> YEYVELAKASLTSAQPQHFYAVVIDATFPYKTNQERYICSLKIVDPTLYLKQQKGAGDASDYATLVLYAKRFEDLPIIHRAGD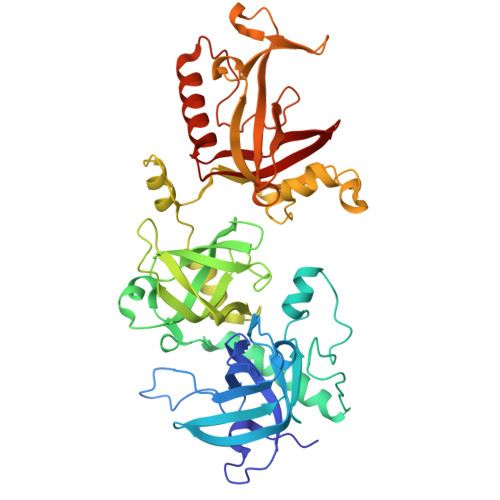IIRVHRATLRLYNGQRQFNANVFYSSSWALFSTDKRSVTQEINNQDAVSDTTPFSFSSKHATIEKNEISILQNLRKWANQYFSSYSVISSDMYTALNKAQAQKGDFDVVAKILQVHELDEYTNELKLKDASGQVFYTLSLKLKFPHVRTGEVVRIRSATYDETSTQKKVLILSHYSNIITFIQSSKLAKELRAKIQDDHSVEVASLKKNVSLNAVVLTEVDKKHAALPSTSLQDLFHHADSDKELQAQDTFRTQFYVTKIEPSDVKEWVKGYDRKTKKSSSLKGASGKGDNIFQVQFLVKDASTQLNNNTYRVLLYTQDGLGANFFNVKADNLHKNADARKKLEDSAELLTKFNSYVDAVVERRNGFYLIKDTKLIY>[8x]MDGSGEQPRGGGPTSSEQIMKTGALLLQGFIQDRAGRMGGEAPELALDPVPQDASTKKLSECLKRI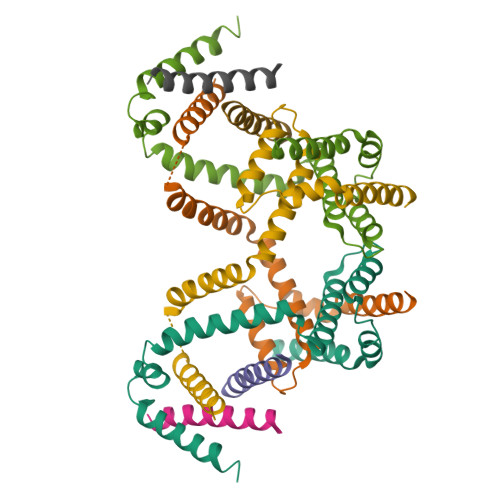GDELDSNMELQRMIAAVDTDSPREVFFRVAADMFSDGNFNWGRVVALFYFASKLVLKALCTKVPELIRTIMGWTLDFLRERLLGWIQDQGGWDGLLSYFGTPTWQTVTIFVAGVLTASLTIWKKMG>MNVGIKGFGAYAPEKIIDNAYFEQFLDTSDEWISKMTGIKERHWADDDQDTSDLAYEASVKAIADAGIQPEDIDMIIVATATGDMPFPTVANMLQERLGTGKVASMDQLAACSGFMYSMITAKQYVQSGDYHNILVVGADKLSKITDLTDRSTAVLFGDGAGAVIIGEVSEGRGIISYEMGSDGTGGKHLYLDKDTGKLKMNGREVFKFAVRIMGDASTRVVEKANLTSDDIDLFIPHQANIRIMESARERLGISKDKMSVSVNKYGNTSAASIP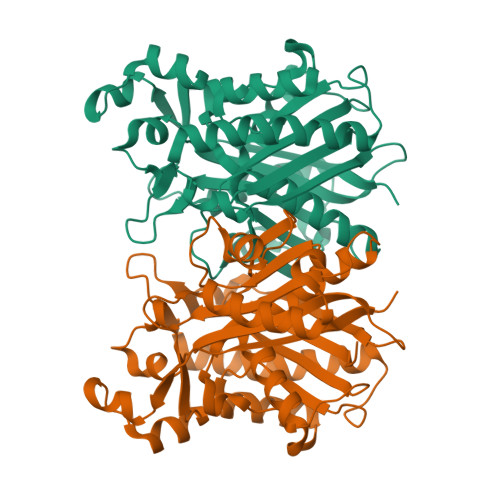LSIDQELKNGKLKDDDTIVLVGFGGGLTWGAMTIKWGK[2x]> AKYTGKCT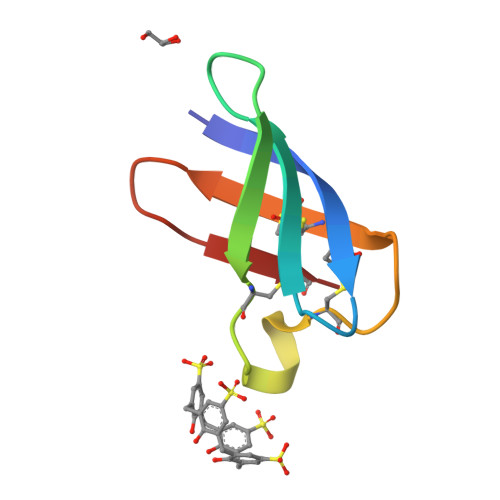KSKNECKYKNDAGKDTFIKCPKFDNKKCTKDNNKCTVDTYNNAVDCD>[2x]MNHKVHHHHHHLQENLYFQGMGAEPQQLHVVFFPIMAHGHMIPTLDIARLFAARNVRATIITTPLNAHTFTKAIEMGKKNGSPTIHLELFKFPAQDVGLPEGCENLEQALGSSLIEKFFKGVGLLREQLEAYLEKTRPN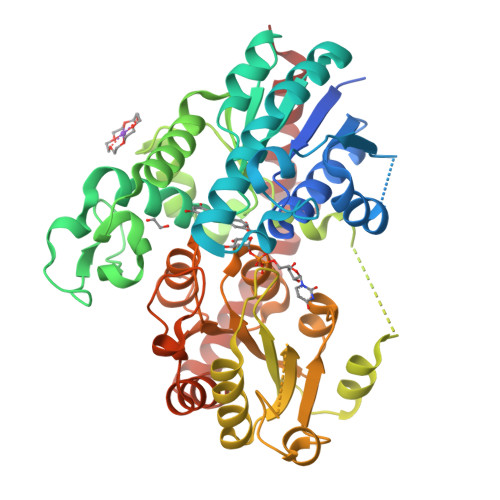CLVADMFFPWATDSAAKFNIPRLVFHGTSFFSLCALEVVRLYEPHKNVSSDEELFSLPLFPHDIKMMRLQLPEDVWKHEKAEGKTRLKLIKESELKSYGVIVNSFYELEPNYAEFFRKELGRRAWNIGPVSLCNRSTEDKAQRGKQTSIDEHECLKWLNSKKKNSVIYICFGSTAHQIAPQLYEIAMALEASGQEFIWVVRNNNNNDDDDDDSWLPRGFEQRVEGKGLIIRGWAPQVLILEHEAIGAFVTHCGWNSTLEGITAGVPMVTWPIFAEQFYNEKLVNQILKIGVPVGANKWSRETSIEDVIKKDAIEKALREIMVGDEAEERRSRAKKLKEMAWKAVEEGGSSYSDLSALIEELRGYHA>AEAGITGTWYN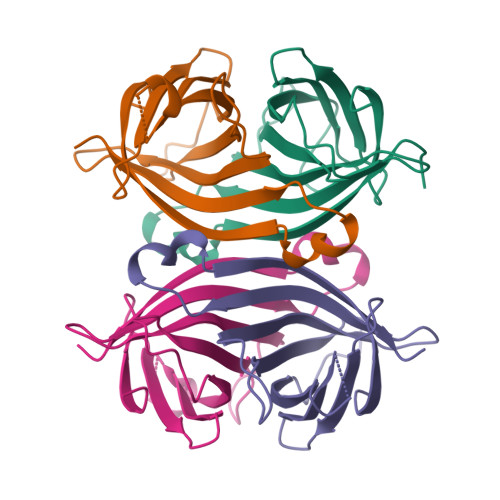QLGSTFIVTAGADGALTGTYESAVGNAESRYVLTGRYDSAPATDGSGTALGWTVAWKNNYRNAHSATTWSGQYVGGAEARINTQWLLTSGTTEANAFKSTLVGHDTFTKVKPSAAS[4x]>MRGSMANINDSKILSLQNRKNTLVDTSGYNAEVSEEGDVQLNPIFPFDFKLGSSGEDRGKVIVTQNENIVYNSMYESFSISFWIRINKWVSNLPGYTIIDSVKNNSGWSIGIISNFLVFTLKQNEDSEQSINFSYDISNNAPGYNKWFFVTVTNNMMGNMKIYINGKLIDTIKVKELTGINFSKTITFEINKIPDTGLITSDSDNINMWIRDFYIFAKELDGKDINILFNSLQYTNVVKDYWGNDLRYNKEYYMVNIDYLNRYMYANSRQIVFNTRRNNNDFNEGYKIIIKRIRGNTNDTRVRGGDILYFDMTINNKAYNLFMKNETMYADNHSTEDIYAIGLREQTKDINDNIIFQIQPMNNTYYYASQIFKSNFNGENISGICSIGTYRFRLGGDWYRHNYLVPTVKQGNYASLLESTSTHWGFVPVSEPGSAWS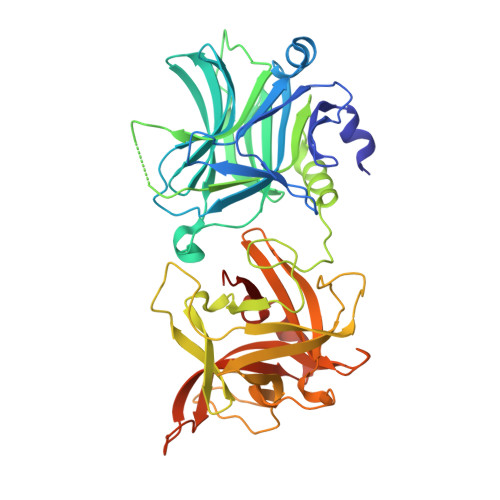HPQFEK[2x]> GGQLQA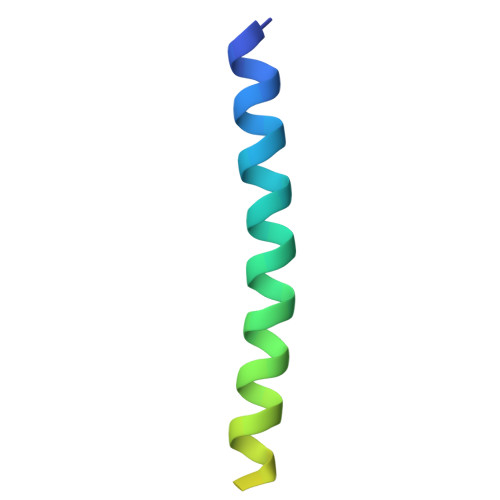AESRYEAQKRITQVFELEILDLYGRLEKDGLLKKLEEEKAEAAEAAEER[(2S)-2-SULFANYL-3-PHENYLPROPANOYL]-GLY-(5-PHENYLPROLINE) | C22 H24 N2 O4 S | 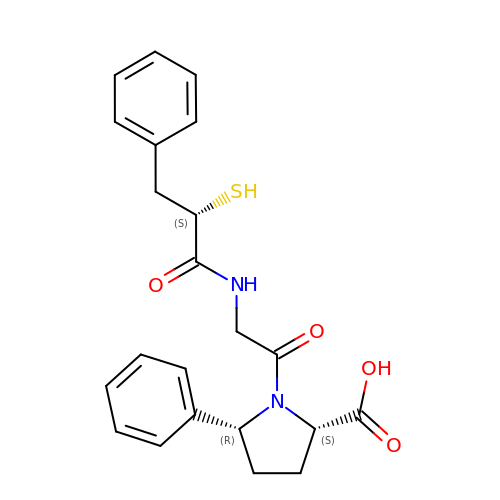ZWDQTNWLXALTOV-QYZOEREBSA-N I-PpoI is a well-characterized intron-encoded homing endonuclease member of the physarum polycephalum slimemold. A large subfamily of one-metal-ion-dependent nucleases consist of histidine-metal (His-Me) nucleases that perform critical tasks in biological pathways such as apoptosis, extracellular defense, intracellular immunity (CRISPR–Cas9), and intron homing (homing endonuclease). Surrounded by two beta sheets and an alpha helix, the His-Me nucleases active sites all contain a single metal ion, a histidine, and an asparagine. The asparagine residue helps to stabilize metal ion binding whereas the strictly conserved histidine is suggested to deprotonate a nearby water for nucleophilic attack toward the scissile phosphate.

Because His98 has been proposed to primarily activate the nucleophilic water, we first mutated His98 to alanine. As expected, cleavage activity of H98A I-PpoI drastically dropped. Furthermore, we found that titrating imidazole in H98A and H78A/H98A I-PpoI partially rescued cleavage activity, similar as observed in Cas9 and EndA nuclease. (D) Structure of H98A I-PpoI active site after 100 mM imidazole for 15 hr following 1 mM Mn2+ soaking for 1800s. Although we tried soaking the H98A I-PpoI crystals in 1 mM Mg/Mn2+ and 100 mM imidazole for 15 h, metal ion binding, imidazole binding, or product formation were not detected, possibly due to the difficulty of imidazole diffusion within the lattice. The results indicate that metal ion binding can be altered by perturbing His98 and possibly water deprotonation, even though the metal ion-binding site and His98 exist 7 Å apart without direct interaction. Our results indicate that perturbing the deprotonation pathway not only affects nucleophilic attack but also metal binding, suggesting that I-PpoI catalyzes DNA catalysis via a concerted mechanism. Moreover, the metal ion was not observed in crystallo when His98 was removed. Without a proper proton acceptor, the metal ion may be prone for dissociation without the reaction proceeding, and thus stable Mg2+ binding was not observed in crystallo without His98.

>[2x]ALTNAQILAVIDSWEETVGQFPVITHHVPLGGGLQGTLHCYEIPLAAPYGVGFAKNGPTRWQYKRTINQVVHRWGSHTVPFLLEPDNINGKTCTASALCHNTRCHNPLHLCWESLDDNKGRNWCPGPNGGCVHAVVCLRQGPLYGPGATVAGPQQRGSHFVV> PVS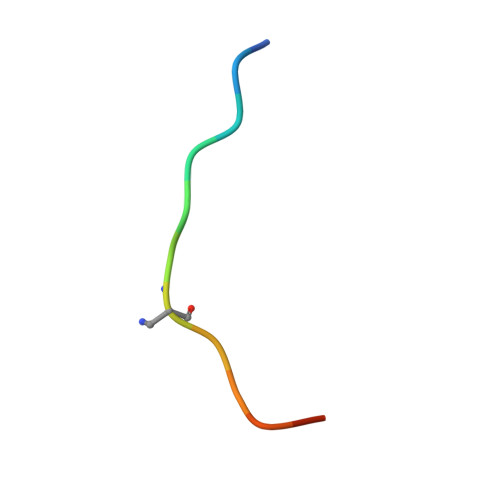VPYASAQSTS>[2x]MDPLTVYKNSVKQQIDSADLLVANLVNENFVLSEKLDTKATEIKQLQKQIDSLNAQVKELKTQTSQQAENSEVIKDLYEYLCNVRVHKSYEDDSGLWFDISQGTHSGGSSDDYSIMDYK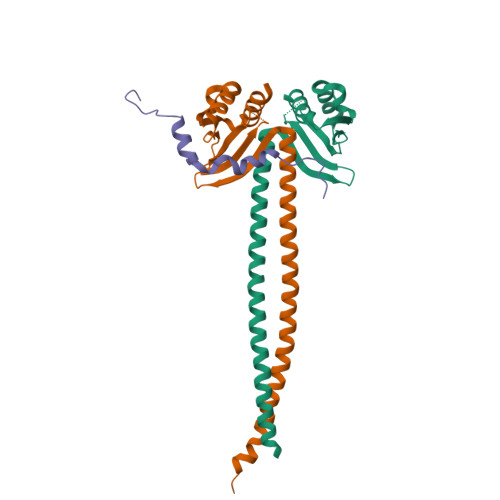LGFVKGQAQVTEVIYAPVLKQRSTEELYSLQSKLPEYLFETLSFPLSSLNQFYNKIAKSLNKKREKKDETE;> QKKRFLPQSVLIKREDEIAFDDFHLDARKVLNDLSATSENPFSSSPNTKKIKSKGKTLEVVPKKKNKKII> SMVAWFAFDPGSAHSD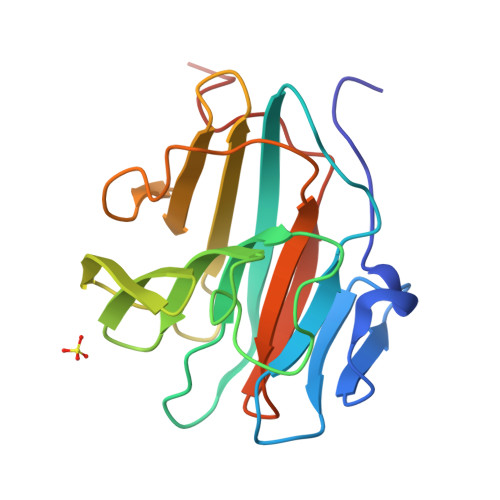IILSNDNLTVTCSSYDDRVVLGKTGFSKGIHYWELTVDRYDNHPDPAFGVARMDVMKDVMLGKDDKAWAMYVDNNRSWFMHNNSHTNRTEGGITKGATIGVLLDFNRKNLTFFINDEQQGPIAFDNVEGLFFPAVSLNRNVQVTLHTGLPVPDFYSSRASIA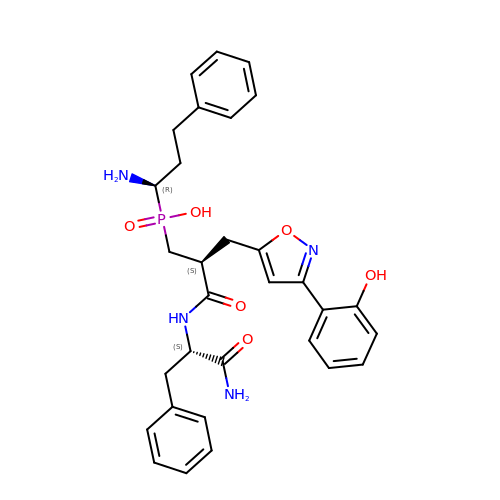[(2~{S})-3-[[(2~{S})-1-azanyl-1-oxidanylidene-3-phenyl-propan-2-yl]amino]-2-[[3-(2-hydroxyphenyl)-1,2-oxazol-5-yl]methyl]-3-oxidanylidene-propyl]-[(1~{R})-1-azanyl-3-phenyl-propyl]phosphinic acid | C31 H35 N4 O6 P | GSWUIYHGTPVQDP-FNHKZSGOSA-N> QNNVPNTFTDPDSGITFNTWGLDEDSPQTQGGFTFGVALPSDALTTDASEFIGYLKCARNDESGWCGISLGGPMTNSLLITAWPHEDTVYTSLRFATGYAMPDVYEGDAEITQVSSSVNSTHFSLIFRCKNCLQWSHGGSSGGASTSGGVLVLGWVQAFDDPGNPTCPEQITLQQHDNGMGIWGAQLNTDAASPSYTDWAAQATKTVTGDCEGPTETSVVGVPVPTGVSFDYIVVGGGAGGIPAADKLSEAGKSVLLIEKGFASTANTGGTLGPEWLEGHDLTRFDVPGLCNQIWVDSKGIACEDTDQMAGCVLGGGTAVNAGLWFKPYSLDWDYLFPDGWKYNDVQPAINRALSRIPGTDAPSTDGKRYYQEGFEVLSKGLAAGGWTSVTANNAPDKKNRTFAHAPFMFAGGERNGPLGTYFQTAKKRNNFDVWLNTSVKRVIREGGHITGVEVEPFRDGGYEGIVPVTKVTGRVILSAGTFGSAKILLRSGIGPEDQLEVVAASEKDGPTMIGNSSWINLPVGYNLDDHLNTDTVISHPDVVFYDFYEAWDDPIESDKNSYLESRTGILAQAAPNIGPMFWEEIVGADGIVRQLQWTARVEGSLGAPNGHTMTMSQYLGRGATSRGRMTITPSLTTIVSDVPYLKDPNDKEAVIQGIINLQNALQNVANLTWLFPNSTITPREYVESMVVSPSNRRSNHWMGTNKLGTDDGRKGGSAVVDLDTRVYGTDNLFVIDASIFPGVPTTNPTSYIVVAAEHASSRILALPDLEPVPKYGQCGGREWTGSFVCADGSTCEYQNEWYSQCL

An oxidative system was recently discovered in which extracellular flavocytochromes, that is, cellobiose dehydrogenases (CDHs), cooperate with copper-dependent lytic polysaccharide monooxygenases (LPMOs)8910111213 to catalyse redox-mediated glycosidic bond cleavage in crystalline cellulose, hemicelluloses and starch. CDHs are large flavocytochromes containing a haem b-binding cytochrome domain (CYT) connected by a long, flexible linker to a flavin adenine dinucleotide (FAD)-binding dehydrogenase domain (DH). The DH domain oxidizes cellobiose at the C1 position to cellobiono-1,5-lactone with reduction of FAD. The ensuing step involves inter-domain electron transfer (IET) from the reduced FAD to CYT haem b, presumably by single electron-transfer (ET) events, followed by ET from CYT to external electron acceptors such as LPMOs.

The crystal structure of MtCDH was determined at 3.2 Å and revealed a closed state in which the CYT domain is docked onto the DH domain in an arrangement that would allow efficient IET from FAD to haem b. In the closed IET-competent state, the haem b propionate-A stretches into the active-site pocket in DH, where the propionate carboxyl group forms an anion–quadrupole interaction with the electropositive edge of the Trp295 benzene ring. Propionate-A engages in an ionic interaction with Arg698, which stabilizes the propionate in its ionized state. The haem b propionate-D is folded away, and a hydrogen bond to Tyr99 in CYT prevents it from interacting directly with the DH active site. The closest edge-to-edge distance between haem b and FAD is 9 Å. This distance is well within the 14-Å limit for efficient electron transfer and is nearly identical to the haem-FMN distance of 9.7 Å in flavocytochrome b2, for which rapid IET has been observed. The MtCDH structure indicates that the haem b propionate-A in CYT interacts with four side chains in DH at the CYT-DH interface, that is, Trp295, Ser298, Met309 and Arg698, a region that we refer to as the propionate-docking site on DH. A channel leads from the surface into the active site of the closed MtCDH molecule. The size of this channel is sufficient (∼11 × 12 Å) to permit substrate entry and product exit while MtCDH remains in the closed IET-competent state. The crystal structure of the closed state of MtCDH offers a favourable association mode between the CYT and DH domains to permit efficient IET.>[2x]EVDCELQPVIEANLSLNQNQLASNGGYISSQLGIRNESCETVKFKYWLSIKGPEGIYFPAKAVVGVDTAQ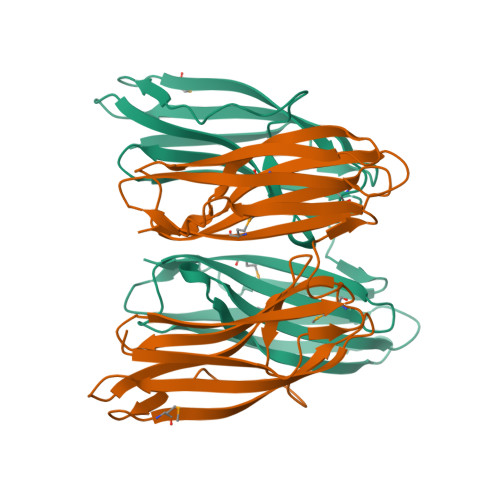QESDALTDGRMLNVTRGFWVPEYMADGKYTVSLQVVAENGKVFKANQEFVKGVDLNSLPELNGLTIDIKNQFGINSVESTGGFVPFTVDLNNGREGEANVEFWMTAVGPDGLIIPVNAREKWVIASGDTYSKVRGINFDKSYPAGEYTINAQVVDIVSGERVEQSMTVVKK Glycogen is the primary storage polysaccharide in bacteria and animals. It is a glucose polymer linked by α-1,4 glucose linkages and branched via α-1,6-linkages, with the latter reaction catalyzed by branching enzymes. In the third step, catalyzed by the branching enzyme (BE), an alpha-1,4 linkage is cleaved, and its reducing end is reattached to make α-1,6 branch points on the polymer. All of the structures have in common a carbohydrate binding module 48 (CBM48) domain n-terminal to the canonical (βα)8 TIM barrel catalytic domain common to all GH13 enzymes and a c-terminal β-sandwich domain common to a number of GH13 enzymes, including the α-amylases, isoamylases, and a number of others.

Herein, we report the structure of M8-bound EcBE, which, to our surprise, identified an additional five new surface glucan binding sites, creating a large glucan surface concentrated on one side of the enzyme. As was the case for all previous malto-oligosaccharide-bound EcBE structures, EcBE with its N-domain removed (the first 113 amino acids of full-length EcBE) was used for crystallization, and soaking these previously grown crystals in high concentrations of M8 was the only path to diffraction-quality M8-bound EcBE crystals. A new EcBE crystal form was used in this case, which has different crystal packing interactions, possibly freeing other regions of the molecule for sugar binding. As was the case for previous structures, there are four unique molecules in the asymmetric unit that provide additional possibilities for sugars to bind without destroying the lattice. However, probably due to the large number of binding sites available on each EcBE molecule, resolution was significantly compromised by M8 soaking, giving a structure of relatively low resolution (3.0 Å). Binding in the five previously identified sites was relatively similar to that seen in the M7-bound EcBE structure for most of the sites, though more glucose units were seen in most of the five sites (compare the 4, 2, 2, 2, and 2 glucose units seen in sites I–V in the M7-bound EcBE structure to the 7, 2, 1, 4, and 3 glucose units seen in the M8-bound EcBE structure). However, M8 binding in site I is quite different from that seen in the M7-bound structure. As shown, three glucose units, not seen in the M7-bound structure, wrap around the 247–264 loop (which connects β1 and α1 of the (α,β)8 central catalytic TIM barrel domain), ending at the entrance to site VII, suggesting that an even longer glucan would span sites I and VII. Remembering that sites I and VII are conserved in only enterobacterial enzymes and the preference of these enzymes for the transfer of longer glucans, it is reasonable to hypothesize that binding from the active site to sites I and VII would provide a binding surface for such longer transferred glucans.

>[4x]GTHLRPYETLGAHADTMDGVTGTRFSVWAPNARRVSVVGQFNYWDGRRHPMRLRKESGIWELFIPGAHNGQLYKYEMIDANGNLRLKSDPYAFEAQMRPETASLICGLPEKVVQTEERKKANQFDAPISIYEVHLGSWRRHTDNNFWLSYRELADQLVPYAKWMGFTHLELLPINEHPFDGSWGYQPTGLYAPTRRFGTRDDFRYFIDAAHAAGLNVILDWVPGHFPTDDFALAEFDGTNLYEHSDPREGYHQDWNTLIYNYGRREVSNFLVGNALYWIERFGIDALRVDAVASMIYRDYSRKEGEWIPNEFGGRENLEAIEFLRNTNRILGEQVSGAVTMAEESTDFPGVSRPQDMGGLGFWYKWNLGWMHDTLDYMKLDPVYRQYHHDKLTFGILYNYTENFVLPLSHDEVVHGKKSILDRMPGDAWQKFANLRAYYGWMWAFPGKKLLFMGNEFAQGREWNHDASLDWHLLEGGDNWHHGVQRLVRDLNLTYRHHKAMHELDFDPYGFEWLVVDDKERSVLIFVRRDKEGNEIIVASNFTPVPRHDYRFGINQPGKWREILNTDSMHYHGSNAGNGGTVHSDEIASHGRQHSLSLTLPPLATIWLVREAE> MKAVIAKNEEQLKDAFYVREEVFVKEQNVPAE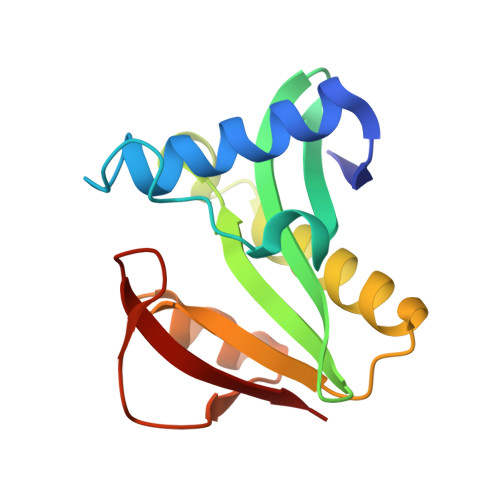EEIDELENESEHIVVYDGEKPVGAGRWRMKDGYGKLERICVLKSHRSAGVGGIIMKALEKAAADGGASGFILNAQTQAVPFYKKHGYRVLSEKEFLDAGIPHLQMMKD>[4x]GSHMMPGEIRPTIGQQMETGDQRFGDLVFRQLAPNVWQHTSYLDMPGFGAVASNGLIVRDGGRVLVVDTAWTDDQTAQILNWI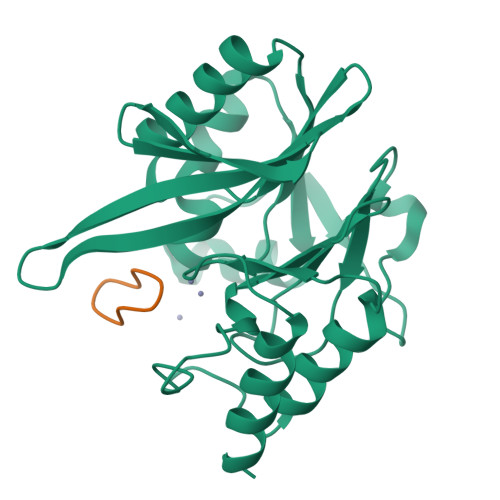KQEINLPVALAVVTHAHQDKMGGMDALHAAGIATYANALSNQLAPQEGMVAAQHSLTFAANGWVEPATAPNFGPLKVFYPGPGHTSDNITVGIDGTDIAFGGCLIKDSKAKSLGNLGDADTEHYAASARAFGAAFPKASMIVMSHSAPDSRAAITHTARMADKLR;>[4x]RRLCPVPE> ERPEPELIRQSWRCVSRSPLEHGTVLFARLFALEPDLLPLFQYNCRQFSSPEDCLSSPEFLDHIRKVMLVIDAAVTNVEDLSSLEEYLASLGRKHRAVGVKLSSFSTVGE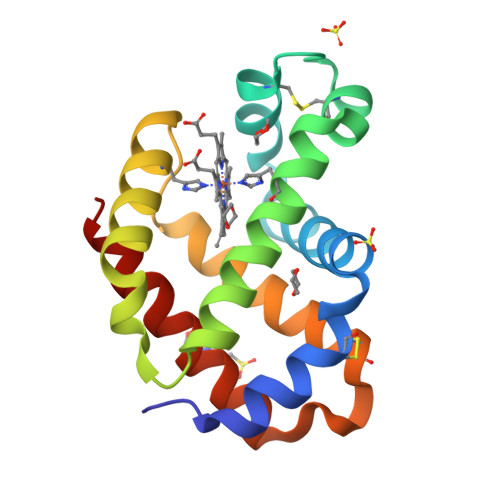SLLYMLEKCLGPAFTPATRAAWSQLYGAVVQAMSRGWD The toxin-coregulated pilus (TCP), an operon-encoded type IVb pilus (T4bP), plays a crucial role in this process, which requires an additional secreted protein, TcpF, encoded on the same TCP operon; however, its mechanisms of secretion and function remain elusive. Here, we demonstrated that TcpF interacts with the minor pilin, TcpB, of TCP and elucidated the crystal structures of TcpB alone and in complex with TcpF. Repetitive TcpA units form the filament structure, whereas TcpB displays multiple functions, such as efficient pilus assembly, pilus retraction, and CTXφ uptake. The structural analyses reveal how TCP recognizes TcpF and its secretory mechanism via TcpB-dependent pilus elongation and retraction.

To clarify the interaction between TcpB and TcpF, we performed cocrystallization experiments with the TcpB-TcpF complex. The initial phases were solved to a resolution of 4.05 Å by molecular replacement (MR) using the reported TcpF structure and TcpB structure determined here (details below) as search models. The three TcpB molecules formed a trimer in an asymmetric unit. In addition, three TcpF molecules were found above the C-terminal domain 3 of TcpB. This feature differed from that of the ETEC CofB-CofJ complex, in which minor pilin CofB interacts with the secreted protein CofJ at a 3:1 molar ratio. Every TcpF molecule was a bilobed structure constituting an NTD and a CTD connected by a short linker, with little interaction between them. These CTDs were spatially separated without direct contact. The structural analysis suggested the existence of a TcpF trimer shaped like a flower with three petals and an N-terminal flexible extension, which partly interacts with the clefts at the interfaces of the TcpB trimer. However, the model building of the N-terminal binding region was unsuccessful due to the relatively low resolution of the present x-ray data. The TcpF trimer formed via an interaction with the NTD, where the interaction surfaces primarily consisted of hydrophobic and aromatic residues, such as Tyr31, Leu32, Ile35, Leu44, Phe98, Leu100, and Phe105, forming a hydrophobic core accompanied by some polar residues making a network of salt bridges between Arg41, Asp97, and Glu108.

>GGELMIKSSNAFDVIELSSQIQRYASLSKINNRTNPILKDNKAKEFKDADLKWLKLENCPTAGDVPTTGNNNDLQDQFIACDADYRKGDLSYFGSQFEFSTYVHPSNPEIQRQIKQVVSYFQYRGMERAFIGDAAGYVISEAKKKGFSAQDYRIVLIEPDRVGYFESNAISYEEFIENPSARENFLLKATKDRTLALAVSLAQTGEIAMQRDGSVAFLEDSELCWDTAAGSAKSCLSVRYDTVGNKTELDLKQIDVVSAKGLSFESDGKTKTPVVSTYETFQDGGRAKTINAIECPTGLNNRFAAVVSSFSTAGQNANFSSESAKDSQGTTQKDGSKGPHALLSGISLNWTLTNKVWDVTASIGIESGILPTSGIDSGSLLRNPKSLSFIAFQWCEN[3x];>[3x]FNDNYSSTSTVYATSNEATDSRGSEHLRYPYLECIKIGMSRDYLENCVKVSFPTSQDMFYDAYPSTESDGAKTRTKEDFSARLLAGDYDSLQKLYIDFYLAQTTFDWEIPTRDQIETLVNYANEGKLSTALNQEYITGRFLTKENGRYDIVNVGGVPDNTPVKLPAIVSKRGLMGTTSVVNAIPNEIYPHIKVYEGTLSRLKPGGAMIAVLEYDVNELSKHGYTNLWDVQFKVLVGVPHAETGVIYDPVYEETVKPYQPSNNLTGKKLYNVSTNDMHNGYKWSNTMFSNSNYKTQILLTKGDGSGVKLYSKAYSENFK>CGCIAATTAGCG[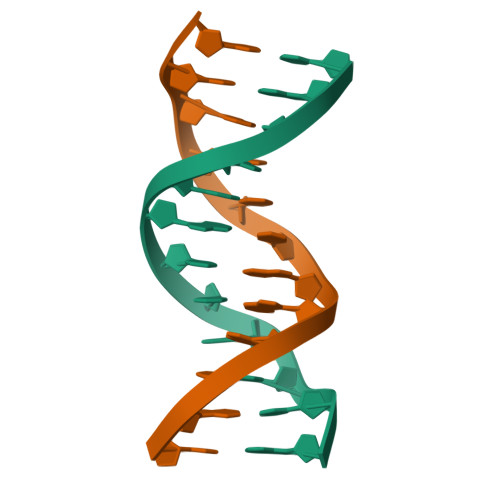2x]5-chloro-N-({(5S)-2-oxo-3-[4-(3-oxomorpholin-4-yl)phenyl]-1,3-oxazolidin-5-yl}methyl)thiophene-2-carboxamide 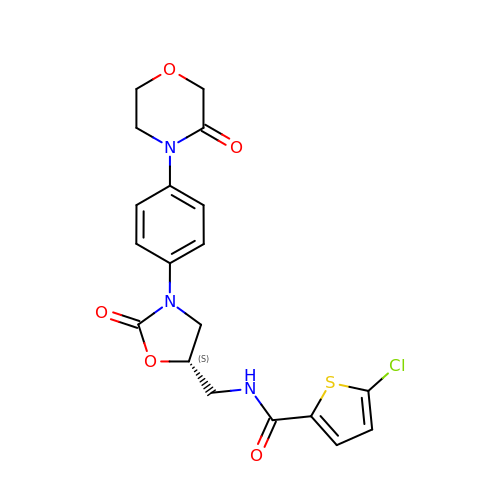| C19 H18 Cl N3 O5 S | KGFYHTZWPPHNLQ-AWEZNQCLSA-N 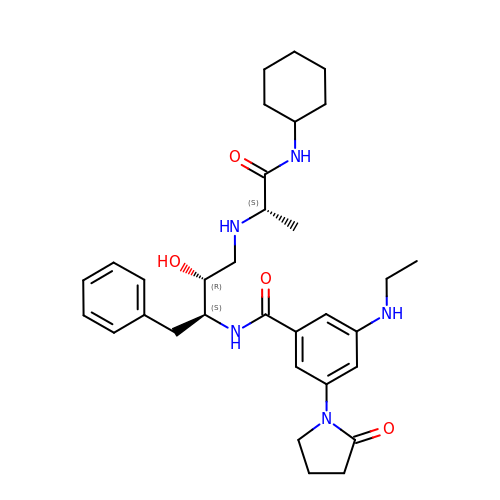N-[(1S,2R)-1-benzyl-3-{[(1S)-2-(cyclohexylamino)-1-methyl-2-oxoethyl]amino}-2-hydroxypropyl]-3-(ethylamino)-5-(2-oxopyrrolidin-1-yl)benzamide | C32 H45 N5 O4 | ARWMRRUIIHCDKG-PWUSVURUSA-N> KETAAAKFERQHMDSSTSAASSSNYCNQMMKSRNLTKDRCKPVNTFVHESLADVQAVCSQKNVACKNGQTNCYQSYSTMSIT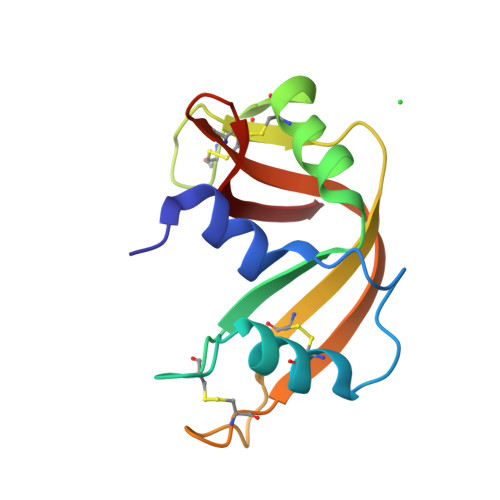DCRETGSSKYPNCAYKTTQANKHAIVACEGNPYVPVHFDASV>GMRPHSALLENMHIEQLARRLPARVQGYPWRLAYSTLEHGTSLKTLYRKSASLDSPVLLVIKDMDNQIFGAYATHPFKFSDHYYGTGETFLYTFSPHFKVFKWSGENSYFINGDISSLELGGGGGRFGLWLDADL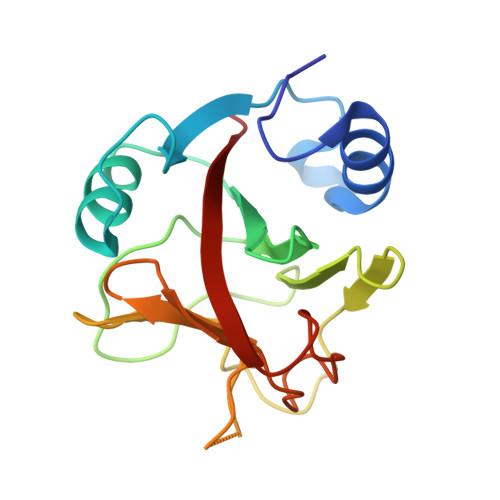YHGRSNSCSTFNNDILSKKEDFIVQDLEVWAFD[6x]>[2x]MGMKHHLLAAFFFISLSPLHAVDATATKNIASPLFQEQMFSLLPVAPDFPKTDFAVSTTTDFVPSKGPWSTTCSEESVFLRSFHTVDLEGKPIELRVGKGGHLYSIQSAIGELVPPQWRHANHKTVSPWNDEVWQAVAVTSDPNKVFVHQSGCYVKPEEPPFYAPCLAQSWSQEDKTFTMLSWGIVPQVTSTLVSEVLYYTRYRFVAPG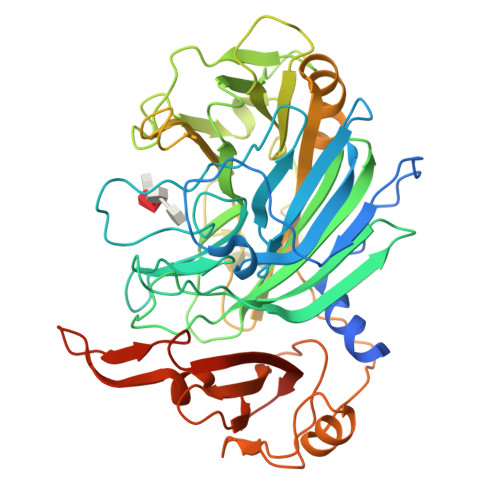VVEVTSGLFDFGKRNYLWLNTPWGGVRQTALGELWIADKSERGTAKWLNPMPRFGAAHDGALDSAGNTGGWMAFAEEGQDPNRYAMGLTFGRDVFPTTGMNSALLPRDKTLIRFGQAGGKETRNYIVAVVIPRLGVISGHGVWWRYYMAFGAFEALKKQCPDWADKTSGGEMVVPSISSETRNFEKCIESGVIPRDATLGSDLSRSHVFSPWPKPEYVPVFAFQLKKDSTWVVTTDPSKYAALGEKDSKGQELYSVAMSFSEIRLLGFTSISSNPSKAAALEHHHHHH>[4x]GHMVDTSGVKIHPAVD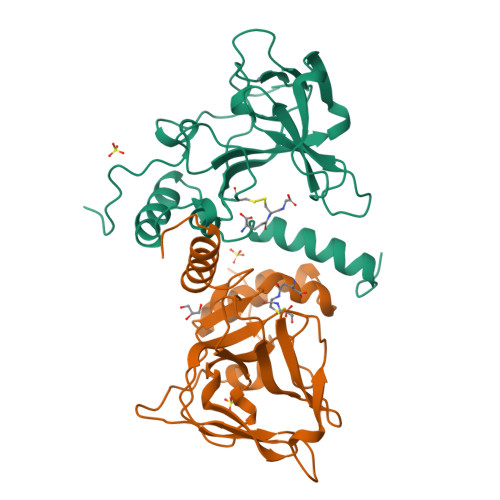NGIKPAQPGFAGGTLHCKCSTNPVRVAVRAQTAHNHVCGCTKCWKPEGAIFSQVAVVGRDALEVLEGAEKLEIVNAEAPIQRHRCRDCGVHMYGRIENRDHPFYGLDFVHTELSDEDGWSAPEFAAFVSSIIESGVDPSRMEAIRARLRELGLEPYDALSPPLMDAIATHIAKRSGALAA>MGSDKIHHHHHHMEMRFFVLGAGSWGTVFAQMLHENGEEVILWARRKEIVDLINVSHTSPYVEESKITVRATNDLEEIKKEDILVIAIPVQYIREHLLRLPVKPSMVLNLSKGIEIKTGKRVSEIVEEILGCPYAVLSGPSHAEEVAKKLPTAVTLAGENSKELQKRISTEYFRVYTCEDVVGVEIAGALKNVIAIAAGILDGFGGWDNAKAALETRGIYEIARFGMFFGADQKTFMGLAGIGDLMVTCNSRYSRNR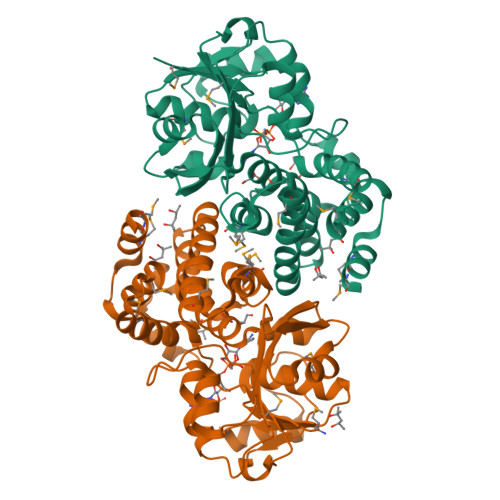RFGELIARGFNPLKLLESSNQVVEGAFTVKAVMKIAKENKIDMPISEEVYRVVYEGKPPLQSMRDLMRRSLKDEFWAS[2x]>GHMRIEVRVDNGRVRVRNGTDRPCRVRVT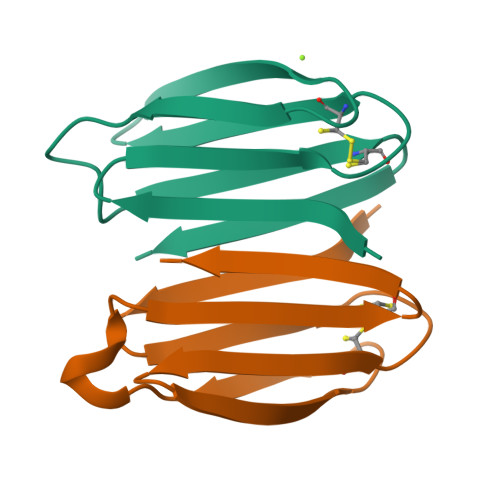AGGETREYTVNPGTELEVELSPEQQNNAEVEVECGNEKYRFQLG[4x]> MDET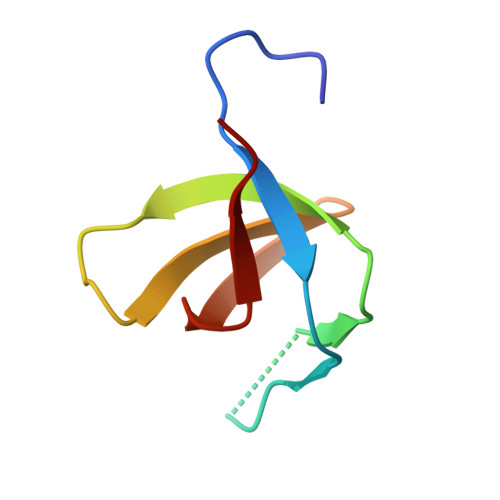GKELLLVLYDYQEKSPRELTLKKGDILTLLNSTNKDWWKVEYNDRQGFIPAAYVKKLD>GSSMKCKFCSREAYIKIHYPKMYLCEEHFKEYFERKVSRTIE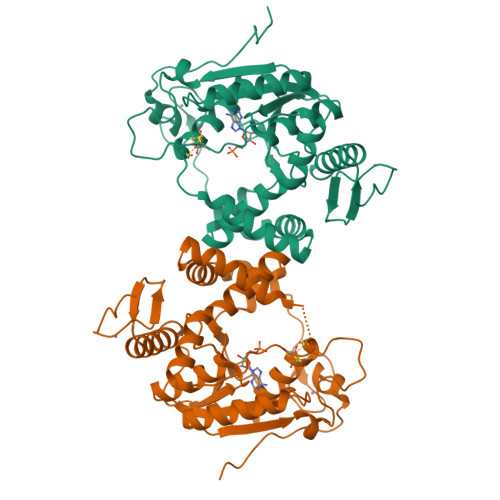RYKLLTKDERILVAVSGGKDSAVTAYVLKKLGYNIECLHINLGISGYSEKSEEYAKKQCKLIGAPLHIVRIKEILGYGIGEVKTRRPPCSYCGLTKRYIMNKFAYDNGFDAIATGHNLDDEASFLLNNILHWNTEYLAKGGPILPQQGKFIKKVKPLYEVTEREVVAYALAVGLEYIVEECPYARGATTLDMKGVLNELEEKRPGTKFNFVRGYLKKKKLFEPEIKEKEIKECKICRMPSSGDICAFCKFWGLKKEINFKVSSTDEEPFGP[2x]> MGSKLPLRPKRSPPVISEEA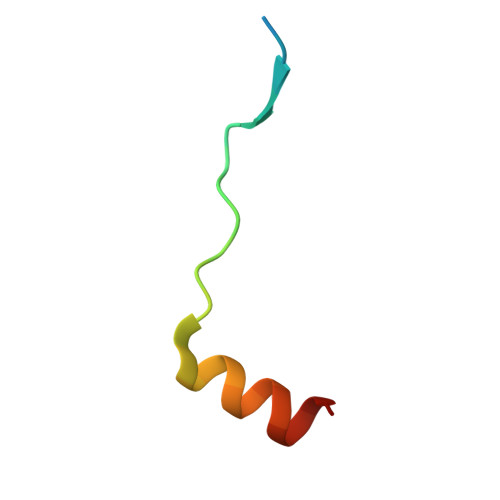AEDVKQYLTI Therefore, the β-xylosidase catalyzing the removal of xylosyl from XDT would play a prominent role in reducing both of the resource waste and pollution to environment. Here we present the crystal structures of LXYL-P1-2 and its complex with XDT. Each monomer comprises three domains as some GH3 members. Sequence alignment of LXYL-P1-2 indicates that Asp300 and Glu529 might act as the catalytic nucleophile and the acid/base residues, respectively.

There are two monomers in the asymmetric unit. The electron density clearly shows the existence of xylose and DT. The xylose adopts a pyranose configuration. It was surprised to found that the glycosidic bond between xylose and DT was broken in both of the monomers. Although the E529Q mutant did not show catalytic activity in the standard enzymatic essay, it may still have weak activity to digest the glycosidic bond of XDT during the crystallization time of one week. Thus, this structure should be regarded as the enzyme/product complex.Fig. 2 a The 2Fo-Fc electron density map (blue, 1.0σ) and Fo-Fc omit map (orange, 3.0σ) for xylose and DT. b Comparison of the overall structure of LXYL-P1-2 in substrate free form (gray) and XDT binding form (green). In the complex, the amide group of Gln529 rotates about 40 degree to form hydrogen bonds to the side-chain OH of Ser466 and the O7 atom of DT. The side-chains of Asp109, Arg174, Lys207, His208, and Asp300 stabilize the xylose by forming hydrogen bonds. Compared with the free enzyme, the only prominent conformational changes in the overall structure upon XDT binding is the movement of loop Ile222-Gln229 with the longest distance of 2.5 Å. DT molecule binds at a pocket formed by several loops: residues 220–232 and 324–328 from domain 1, residues 379–383 which links domain 1 and 2, and residues 446–450 and 529–530 from domain 2. The hydrophobic environment, contributed by Leu220, Ile222, Ile224, Val227, Ile232, Phe324, Leu325, Ala327, Leu328, Ile379, Thr383, and Ala447 form the hydrophobic wall of DT binding pocket.

>MFPARLSLAVLFSVSPALAYFSGLGLGSERSIFRRDLNSTGDESNSTQWPAPLANGGKSWASAFKKAKATVTEMTVEELANITSGVIGLCSGVTGAVTRLGIPEFCLQDGPIGPRGVHGSSQFPAGLTVAATWDRTLMYARARGMGQEFHDQGVHLALAPVTGGPLGRTPLNGRGWEGTFADPYACGEASYLSVKGLTDAGVATVSKHWIAYEQETSRNLYIDIDGVSQADIQLPISSNVDDLTMHELYMWSFAEAVRAGTNHIMCSYNRINNTHSCSNAKGLNQLLKTELNFQGGVVSDWGGQWDSVPAAENGLDVAMPGKGFLGALGDFWGATLVELINNGTVSEDLVRDKAVRILTGYYYLGQDTNPPPPFVYNTIGAPTLNATSGYRNVRKPGTAELIKEIGSASVTLLKNTGSLPLKHPQRIAVLGNDATYNVLGPNACGLANSACDIDNLNGTLTTGGGSGSALSPYTITPLEALQKRAIEDNAEIAAVVANSNTTTGAEDAIAALLPDADVTFVFLNRYSEQGADAPDFSLGGDGDNLMDLAVTYSSNVVVVIHTTGVVDIEKWADNPNVTAILVAYLPGQEAGNSLVPVLYGDVAPSGKLPWTWGKSIDDYVPNGVVYTDAYSPQSNFTEGVFIDYRWFDKMGITPRYEFGFGLSYTTFTYSNLIVDHGRWAKDYSSVMETAEPFAEWDGTNSLYDVIFTVFATITNTGNLTGSEVAQLYISIPGDNQPVRQLRGFDKIKDLPVGDSAVVTFPIRRKDVSSWSVVDQLWYVPNGDFLISVGGSSRDLPLNTTWTPHHHHHH[2x]>[13x]PITGSMDTAYANSTQEETFLTSTLCLYYPTEAATEINDNSWKDTLSQLFLTKGWPTGSVYFKEYTDIASFSVDPQLYCDYNVVLM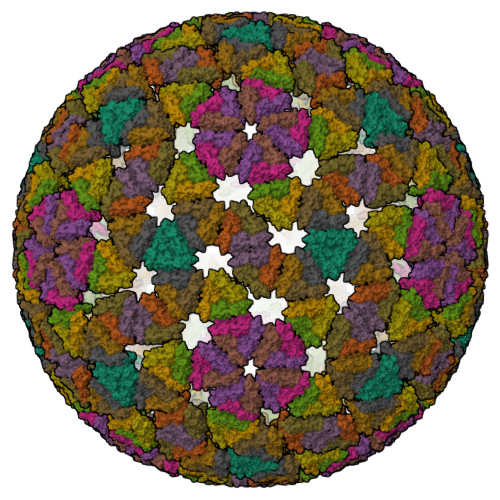KYDATLQLDMSELADLILNEWLCNPMDITLYYYQQTDEANKWISMGSSCTIKVCPLNTQTLGIGCLTTDTATFEEVATAEKLVITDVVDGVNHKLDVTTATCTIRNCKKLGPRENVAVIQVGGSDVLDITADPTTAPQTERMMRINWKKWWQVFYTVVDYVNQIIQAMSK>MEEPEEPADSGQSLVPVYIYSPEYVSMCDSLAKIPKRASMVHSLIEAYALHKQMRIVKPKVASMEEMATFHTDAYLQHLQKVSQEGDDDHPDSIEYGLGYDCPATEGIFDYAAAIGGATITAAQCLIDGMCKVAINWSGGWHHAKKDEASGFCYLNDAVLGILRLRRKFERILYVDLDLHHGDGVEDAFSFTSKVMTVSLHKFSPGFFPGTGDVSDVGLGKGRYYSVNVPIQDGIQDEKYYQICESVLKEVYQAFNPKAVVLQLGADTIAGDPMCSFNMTPVGIGKCLKYILQWQLATLILGGGGYNLANTARCWTYLTGVILGKTLSSEIPDHEFFTAYGPDYVL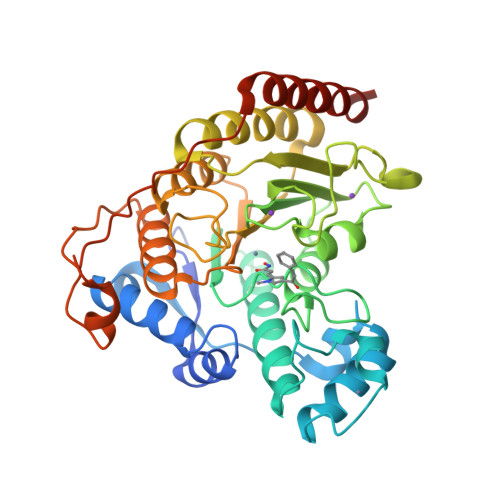EITPSCRPDRNEPHRIQQILNYIKGNLKHVVIEGRSHHHHHH[3x]> MEKSFVITDP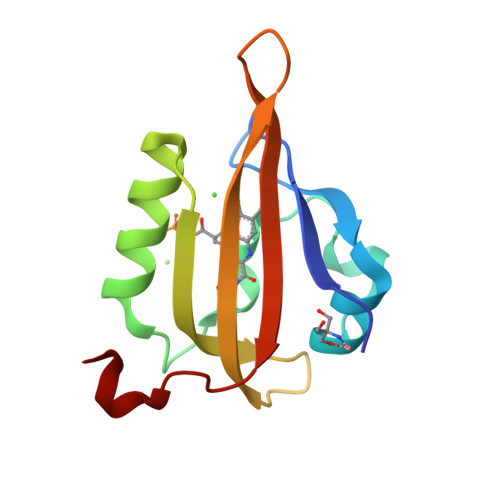RLPDNPIIFASDGFLELTEYSREEILGRNGRFLQGPETDQATVQKIRDAIRDQREITVQLINYTKSGKKFWNLLHLQPMRDQKGELQYFIGVQLDGEFIPNPLLG>[4x]GMNQNKITAGGLEFLVRFAAPTDRLKINDLMIDTARWLKESGSTQWSDILHGFDVHNIEQRIELGE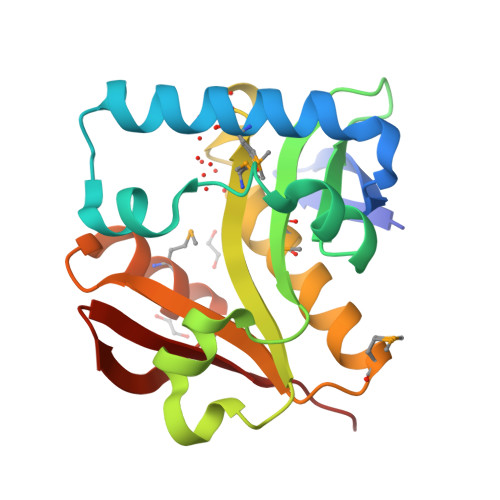VALFETEAGALAGAMIIRKTPSDWDTDLWEDLAIDKAYYLHRIMVSRAFSGISLSKQMIYFAEKLGIEMSVPFIRLDCIESNETLNQMYVRYGFQFSGKKNGFYLYQKELSQK ethyl 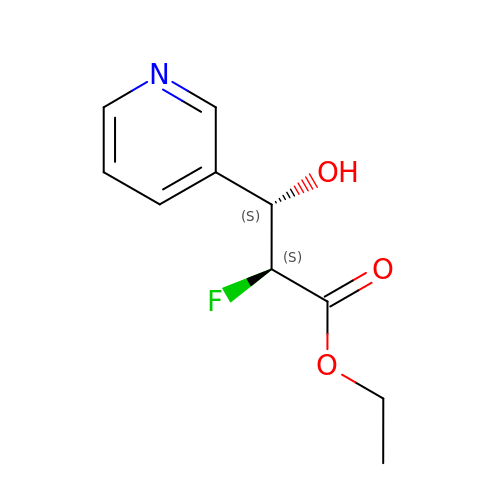(2S,3S)-2-fluoro-3-hydroxy-3-(pyridin-3-yl)propanoate | C10 H12 F N O3 | WQTYAHVCEJEKSU-IUCAKERBSA-N5-[4-(morpholin-4-ylmethyl)phenyl]-3-(1-propan-2-yl-1,2,3-triazol-4-yl)pyridin-2-amine | C21 H26 N6 O | 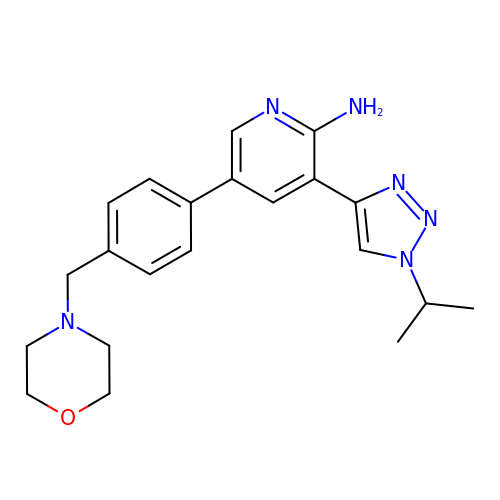CFVWLNQPGCBNKV-UHFFFAOYSA-N> GMADPSLHHEAQPLKFIAVDYSPESCTHSPESSTITLTFDHRGGSRWRSTTRFQYGTFSSLIQCPKGNTSGLNFNIYLSSLEGDKSQDEIDFEFLGKDKRIVQTNYYTAGTGNREAIHDLGFDCSDGFHEYVIKWGPDLIQWLIDGKVIRSVRADGEGFPQKPMFLYASVWDASYIDEGRWTGPYVGSDAPYI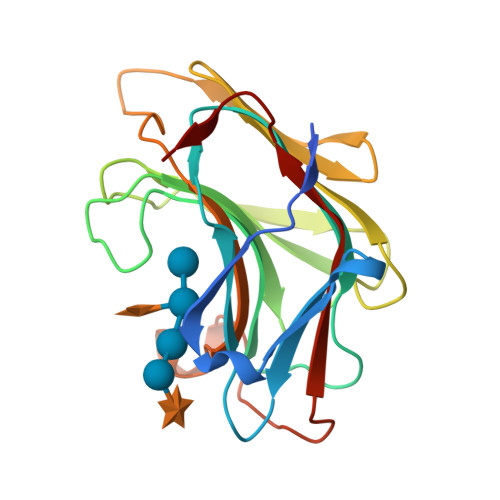CLYKNVNVPVGTAVE> DPMDLHMMNCELLATCSALGYLEGDTYHKEPDCLESVKDLIRYLRHEDETRDVRQQLGAAQILQSDLLPILTQHHQDKPLFDAVIRLMVNLTQPALLCFGNLPKEPSFRHHFLQVLTYLQAYKEAFASEKAFGVLSETLYELLQLGWEERQE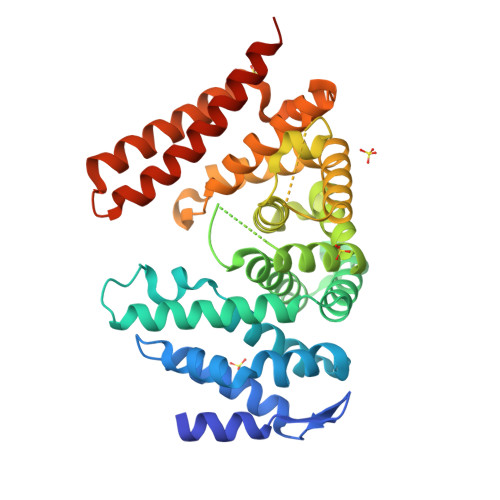EDNLLIERILLLVRNILHVPADLDQEKKIDDDASAHDQLLWAIHLSGLDDLLLFLASSSAEEQWSLHVLEIVSLMFRDQNPEQLAGVGGSTGSTQRRSALNVRLFLRDFCSEFLENCYNRLMGSVKDHLLREKAQQHDETYYMWALAFFMAFNRAASFRPGLVSETLSVRTFHFIEQNLTNYYEMMLTDRKEAASWARRMHLALKAYQELLATVNEMDISPDEAVRE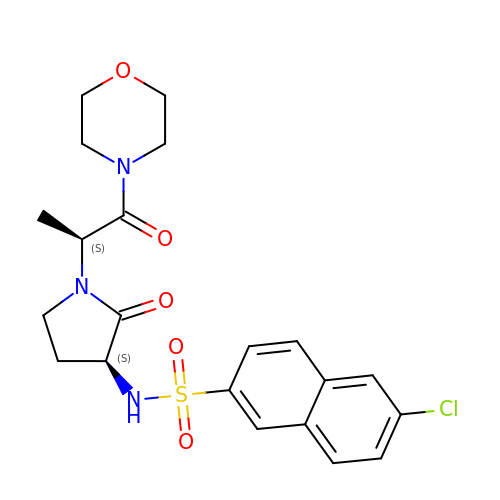6-CHLORO-N-{(3S)-1-[(1S)-1-METHYL-2-(4-MORPHOLINYL)-2-OXO ETHYL]-2-OXO-3-PYRROLIDINYL}-2-NAPHTHALENESULFONAMIDE | C21 H24 Cl N3 O5 S | ICLOZQFWTRAYPX-LIRRHRJNSA-N> MSPLSGSLAPLNMKGLVKFQDVSFAYPNHPNVQVLQGLTFTLYPGKVTALVGPNGSGKSTVAALLQNLYQPTGGKVLLDGEPLVQYDHHYLHTQVAAVGQEPLLFGRSFRENIAYGLTRTPTMEEITAVAMESGAHDFISGFPQGYDTEVGETGNQLSGGQRQAVALARALIRKPRLLILDNATSALAAGNQLRVQRLLYESPEWASRTVLLITQQLSLAERAHHILFLKEGSVCEQGTHLQLMERGGCYRSMVEALAAPSDAAAHHHHHH

Life depends on transport systems that shuttle ions and molecules across cell membranes. Interestingly, the two composite ATP-binding sites are functionally non-equivalent. Membrane transport via alternating access can occur either uni- or bidirectionally.

yielding two copies of the D-loop mutation in the homodimeric state. polarization-based competition assay showed that the affinities for ATP and ADP of isolated wt and D-loop (D651A) mutant rat TAP1-NBD are similar. the crystal structure of Walker B/D-loop double mutant rat TAP1-NBD. form the canonical NBD sandwich interface. asymmetric unit, reveals two significant differences. re-organization, the C-terminal regions slide with respect to each other. key interactions for the D-loop aspartate. γ-phosphate, backbone of A649 and A651, and N654 side chain. overall D-loop and Walker A positions are essentially unaffected. flexibility of the D-loop destabilize the NBD dimer and precludes ATP hydrolysis.>[3x]MFSKFFIERPVFASVVAIIISLAGAIGLTNLPIEQYPSLTPPTVKVSATYTGADAQTIASTVASPIEDAINGADNMIYMDSTSSSSGTMSLTVYFDIGTDPDQATIDVNNRISAATAKMPDAVKKLGVTVRKTSSTTLAAISMYSSDGSMSAVDVYNYITLNVLDELKRVPGVGDANAIGNRNYSLRIWLKPDLLNKFGITATDVISAVNDQNAQYATGKIGEEPVTQKSPYVYSITMQGRLQNPSEFENIILRTNN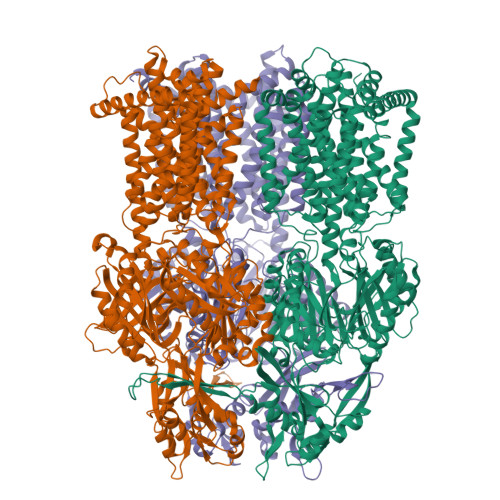DGSFLRLKDVADVEIGSQQYSSQGRLNGNDAVPIMINLQSGANALHTAELVQAKMQELSKNFPKGLTYKIPYDTTKFVIESIKEVVKTFVEALILVIIVMYMFLKNFRATLIPMIAVPVSLLGTFAGLYVLGFSINLLTLFALILAIGIVVDDAIIVVENIDRILHENEQISVKDAAIQAMQEVSSPVISIVLVLCAVFVPVSFISGFVGEIQRQFALTLAISVTISGFVALTLTPSLCALFLRRNEGEPFKFVKKFNDFFDWSTSVFSAGVAYILKRTIRFVLIFCIMLGAIFYLYKAVPNSLVPEEDQGLMISIINLPSASALHRTISEVDHISQEVLKTNGVKDAMAMIGFDLFTSSLKENAAAMFIGLQDWKDRNVSADQIIAELNKKFAFDRNASSVFIGLPPIPGLSITGGFEMYVQNKSGKSYDEIQKDVNKLVAAANQRKELSRVRTTLDTTFPQYKLIIDRDKLKHYNLNMQDVFNTMNATIGTYYVNDFSMLGKNFQVNIRAKGDFRNTQDALKNIFVRSNDGKMIPLDSFLTLQRSSGPDDVKRFNLFPAAQVQGQPAPGYTSGQAIEAIAQVAKETLGDDYSIAWSGSAYQEVSSKGTASYAFALGMIFVFLILAAQYERWLIPLAVVTAVPFAVFGSFLLVYLRGFSNDIYFQTGLLLLIGLSAKNAILIVEFAMEERFKKGKGVFEAAVAAAKLRFRPIIMTSLAFTFGVLPMIFATGAGSASRHSLGTGLIGGMIAASTLAIFFVPLFFYLLENFNEWLDKKRGKVHE> GIQGLAKLIADVAPSAIRENDIKSYFGRKVAIDASMSIYQFLIAVRQGGDVLQNEEGETTSHLMGMFYRTIRMMENGIKPVYVFDGKPPQLKSGELAKRSERRAEAEKQLQQAQAAGAEQEVEKFTKRLVKVTKQHNDECKHLLSLMGIPYLDAPSEAEASCAALVKAGKVYAAATEDMDCLTFGSPVLMRHLTASEAKKLPIQEFHLSRILQELGLNQEQFVDLCILLGSDYCESIRGIGPKRAVDLIQKHKSIEEIVRRLDPNKYPVPENWLHKEAHQ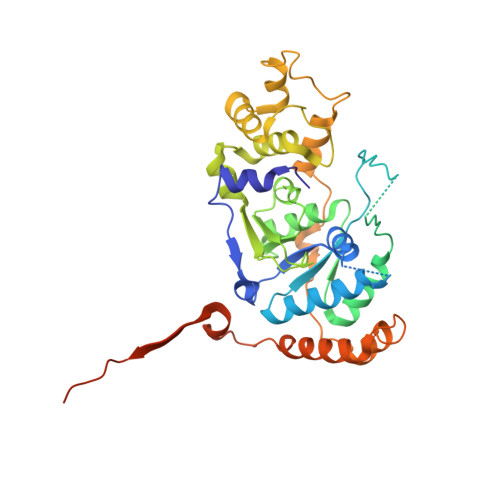LFLEPEVLDPESVELKWSEPNEEELIKFMCGEKQFSEERIRSGVKRLSKSRQGSTQGRLDDFFKVTGSLSSAKRKEPEPKGSTKKKAKTGAAGKFKRGK>MNYLNNIRIENPLTICYTNDVVKNFTANGLLSIGASPAMSEAPEEAEEFYKVAQALLINIGTLTAQNEQDIIAIAQTANEAGLPIVFDPVAVGASTYRKQFCKLLL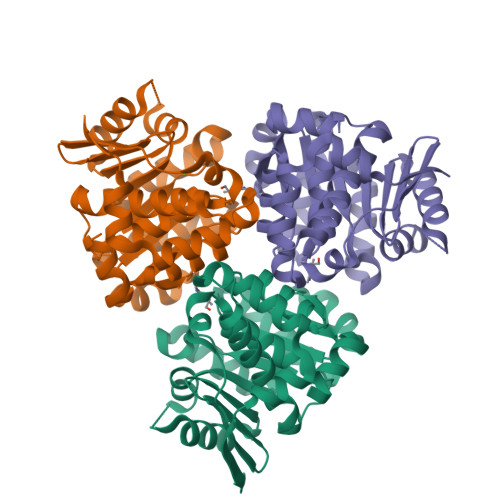KSAKVSVIKGNASEILALIDDTATMKGTDSDANLDAVTIAKKAYAIYKTAIVITGKEDVIVQGDKAIVLANGSPLLARVTGAGCLLGGIIAGFLFRETEPDIEALIEAVSVFNIAAEVAAENENCGGPGTFSPLLLDTLYHLNETTYQQRIRIQEVEENLYQQSGHHHHHH[6x]> MHMEGEYIKLKVIGQDSSEIHFKVKMTTHLKKLKESYCQRQG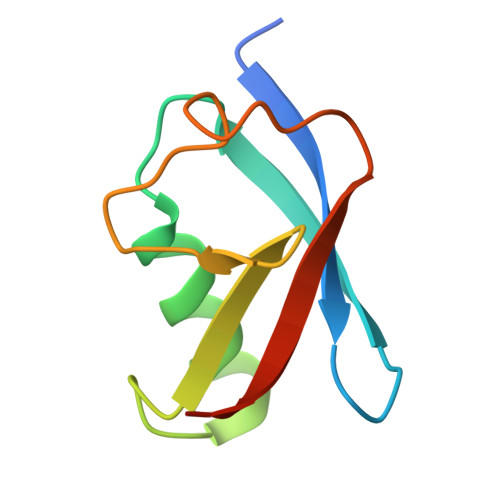VPMNSLRFLFEGQRIADNHTPKELGMEEEDVIEVYQEQTGG>VGPKTGEENQVLVPNLNPTPENLEVVGDGFKITSSINLVGEEEADENAVNALREFLTANNIEINSENDPNSTTLIIGEVDDDIPELDEALNGTTAENLKEEGYALVSNDGKIAIEGKDGDGTFYGVQTFKQLVKESNIPEVNITDYPTVSARGIVEGFYGTPWTHQDRLDQIKFYGENKLNTYIYAPKDDPYHREKWREPYPESEMQRMQELINASAENKVDFVFGISPGIDIRFDGDAGEEDFNHLITKAESLYDMGVRSFAIYWDDIQDKSAAKHAQVLNRFNEEFVKAKGDVKPLITCPTEYDTGAMVSNGQPRAYTRIFAETVDPSIEVMWTGPGVVTNEIPLSDAQLISGIYDRNMAVWWNYPVTDYFKGKLALGPMHGLDKGLNQYVDFFTVNPMEHAELSKISIHTAADYSWNMDNYDYDKAWNRAIDMLYGDLAEDMKVFANHSTRMDNKTWAKSGREDAPELRAKMDELWNKLSSKEDASALIEELYGEFARMEEACNNLKANLPEVALEECSRQLDELITLAQGDKASLDMIVAQLNEDTEAYESAKEIAQNKLNTALSSFAVISEKVAQSFIQEALSFDLTLI[2x]

Posttranslational modification of metazoan nucleocytoplasmic proteins with N-acetylglucosamine (O-GlcNAc) is essential, dynamic, and inducible and can compete with protein phosphorylation in signal transduction. The O-GlcNAc modification is removed by a single enzyme termed O-GlcNAcase (OGA) (Gao et al., 2001). Inhibitors of O-GlcNAcase, the enzyme removing O-GlcNAc, are useful tools for studying the role of O-GlcNAc in a range of cellular processes. Previously reported compounds showed undesirable inhibition of the human lysosomal hexosaminidases, and there has been no direct evidence of the cell penetration of these compounds. This work reports derivatives of the GlcNAcstatin scaffold, showing potent inhibition of human O-GlcNAcase with up to 900,000-fold weaker inhibition of the lysosomal hexosaminidases.

The β-hexosaminidases have a narrower (difference of approximately 1.4 Å) and shallower (difference of approximately 5.0 Å) pocket than the OGA enzymes. Interestingly, a cysteine residue is located at the bottom of the hOGA active site (Cys215). In an attempt to generate a potent, selective hOGA “suicide” inhibitor, the N-acyl group of GlcNAcstatin D was extended and modified to contain thiol-reactive groups that could irreversibly react with the cysteine located in a pocket at the bottom of the active site. GlcNAcstatin F carries a 3-mercaptopropanamide side chain and GlcNAcstatin G a penta-2,4-dienamide derivative, both potentially able to react with the hOGA Cys215. The extension of the N-propionyl side chain of GlcNAcstatin D with an additional thiol group (GlcNAcstatin F) increases selectivity for hOGA to 1000-fold, showing that the elongated N-acyl substitution abolishes the binding of the compound to hHexA/B. The molecular basis of the increased selectivity of the new GlcNAcstatin derivatives was investigated by X-ray crystallography using the CpOGA V331C mutant that perfectly mimics the hOGA active site (Dorfmueller et al., 2009). The CpOGA-V331C GlcNAcstatin F complex (2.5 Å resolution) reveals that the inhibitor-binding mode is similar to the previously reported GlcNAcstatin C/D complexes (Dorfmueller et al., 2006, 2009). The 3-mercaptopropanamide moiety points straight into the pocket of the active site, whereas all hydrogen bonds seen in the GlcNAcstatin C/D complexes are conserved. Interestingly, the sulfhydryl group of GlcNAcstatin F approaches the active site cysteine (Cys215 in hOGA, equivalent to Cys331 in the V331C-CpOGA mutant) to within 3.5 Å, although the side chain thiol points away from the inhibitor, and no disulfide bond is formed, in agreement with the absence of time-dependent inhibition.> MALRGTVTDFSGFDGRADAEVLRKAMKGLGTDEDSILNLLTARSNAQRQQIAEEFKTLFGRDLVNDMKSELAGKFEKLIVALMKPSRLYDAYELKHALKGAGTDEKVLTEIIASRTPEELRAIKQAY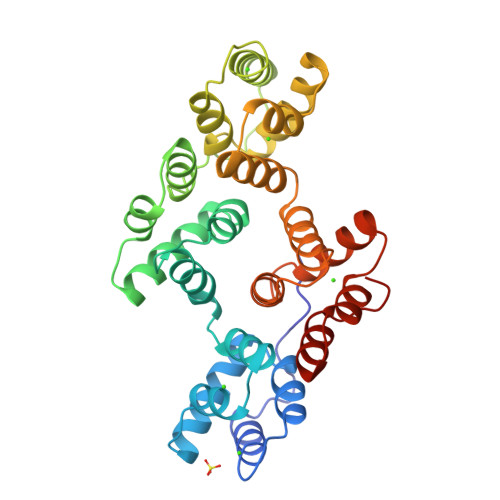EEEYGSNLEDDVVGDTSGYYQRMLVVLLQANRDPDTAIDDAQVELDAQALFQAGELKWGTDEEKFITILGTRSVSHLRRVFDKYMTISGFQIEETIDRETSGNLENLLLAVVKSIRSIPAYLAETLYYAMKGAGTDDHTLIRVIVSRSEIDLFNIRKEFRKNFATSLYSMIKGDTSGDYKKALLLLCGGEDD>MAGARRLELGEALALGSGWRHVCHALLYAPDPGMLFGRIPLRYAILMQMRFDGRLGFPGGFVDTQDRSLEDGLNRELREELGEAAAAFRVERTDYRSSHVGSGPRVVAHFYAKRLTLEELLAVEAGATRAKDH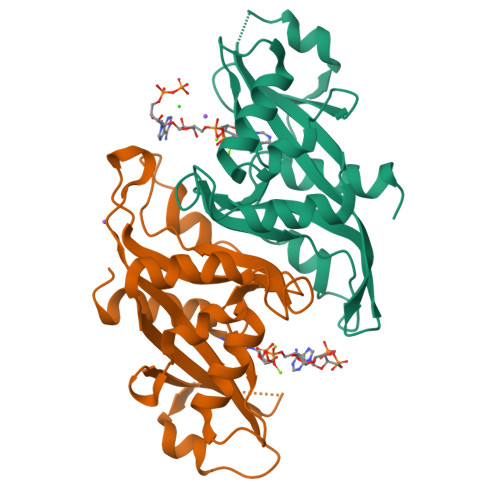GLEVLGLVRVPLYTLRDGVGGLPTFLENSFIGSAREQLLEALQDLGLLQSGSISGLKIPAHH[2x]>VDLEKIPIEEVFQQLKCSREGLTTQEGEDRIQIFGPNKLEEKKESKLLKFLGFMWNPLSWVMEMAAIMAIALANGDGRPPDWQDFVGIICLLVINSTISFIEENNAGNAAAALMAGLAPKTKVLRDGKWSEQEAAILVPGDIVSIKLGDIIPADARLLEGDPLKVDQSALTGESLPVTKHPGQEVFSGSTCKQGEIEAVVIATGVHTFFGKAAHLVDSTNQVGHFQKVLTAIGNFCICSIAIGMVIEIIVMYPIQRRKYRDGIDNLLVLLIGGIPIAMPTVLSVTMAIGSHRLSQQGAITKRMTAIEEMAGMDVLCSDKTGTLTLNKLSVDKNLVEVFCKGVEKDQVLLFAAMASRVENQDAIDAAMVGMLADPKEARAGIREVHFLPFNPVDKRTALTYIDGSGNWHRVSKGAPEQILELAKASNDLSKKVLSIIDKYAERGLRSLAVARQVVPEKTKESPGAPWEFVGLLPLFDPPRHDSAETIRRALNLGVNVKMITGDQLAIGKETGRRLGMGTNMYPSSALLGTHKDANLASIPVEELIEKADGFAGVFPEHKYEIVKKLQERKHIVGMTGDGVNDAPALKKADIGIAVADATDAARGASDIVLTEPGLSVIISAVLTSRAIFQRMKNYTIYAVSITIRIVFGFMLIALIWEFDFSAFMVLIIAILNDGTIMTISKDRVKPSPTP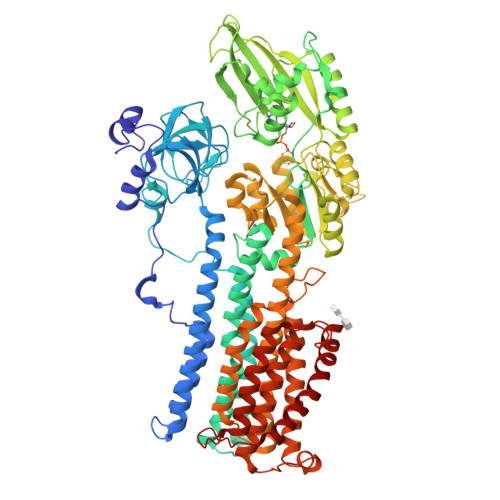DSWKLKEIFATGVVLGGYQAIMTVIFFWAAHKTDFFSDTFGVRSIRDNNHELMGAVYLQVSIISQALIFVTRSRSWSFVERPGALLMIAFLIAQLIATLIAVYANWEFAKIRGIGWGWAGVIWLYSIVTYFPLDVFKFAIRYI[2x]>[4x]KHSL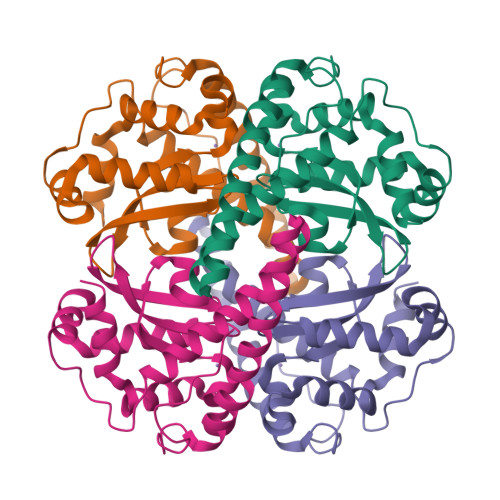PDLPYDYGALEPHINAQIMQLHHSKHHAAYVNNLNVTEEKYQEALAKGDVTAQIALQPALKFNGGGHINHSIFWTNLSPNGGGEPKGELLEAIKRDFGSFDKFKEKLTAASVGVQGSGWGWLGFNKERGHLQIAACPNQDPLQGTTGLIPLLGIDVWEHAYFLQYKNVRPDYLKAIWNVINWENVTERYMACKK> VADVV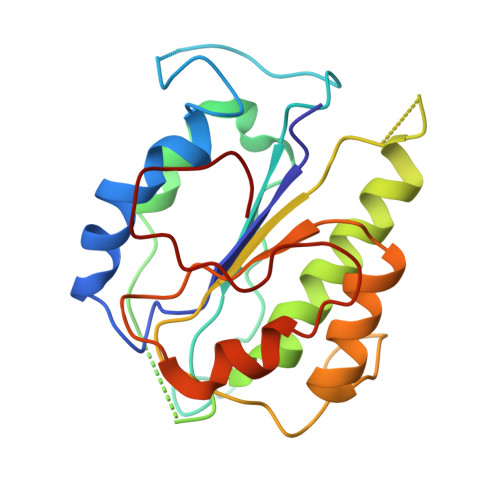FVIEGTANLGPYFEELRKHYLLPAIEYFNGGPPAETDFGGDYGGTQYSLVVFNTVDCAPESYVQCHAPTSSAYEFVTWLDGIKFMGGGGESCSLIAEGLSTALQLFDDFKKMREQIGQTHRVCLLICNSPPYLLPAVESTTYSGCTTESLVQKIGERGIHFSIVSPRKLPALRLLFEKAAPPALLEPLQQPADVSQD>CGCXAATTCGCG[2x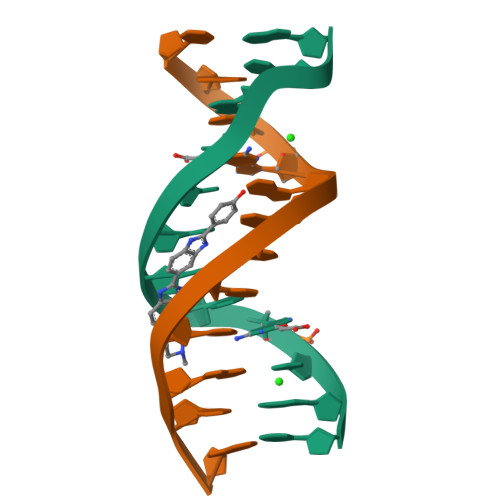]N-ACETYLALANINE | C5 H9 N O3 | 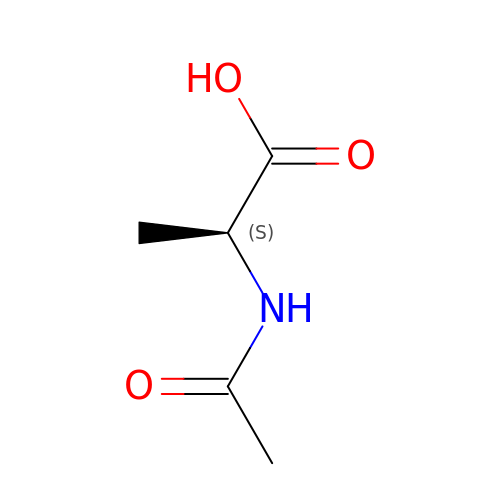KTHDTJVBEPMMGL-VKHMYHEASA-N>[2x]MFDNLTDRLSRTLRNISGRGRLTEDNVKDTLREVRMALLEADVALPVVREFINRVKEKAVGHEVNKSLTPGQEFVKIVRNELVAAMGEENQTLNLAAQPPAVVLMAGLQGAGKTTSVGKLGKFLREKHKKKVLVVSADVYRPAAIKQLETLAEQVGVDFFPSDVGQKPVDIVNAALKEAKLKFYDVLLVDTAGRLHVDEAMMDEIKQVHASINPVETLFVVDAMTGQDAANTAKAFNEALPLTGVVLTKVDGDARGGAALSIRHIT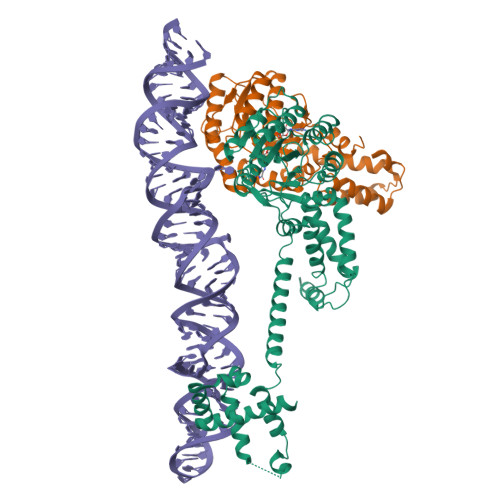GKPIKFLGVGEKTEALEPFHPDRIASRILGMGDVLSLIEDIESKVDRAQAEKLASKLKKGDGFDLNDFLEQLRQMKNMGGMASLMGKLPGMGQIPDNVKSQMDDKVLVRMEAIINSMTMKERAKPEIIKGSRKRRIAAGSGMQVQDVNRLLKQFDDMQRMMKKMKKG;>FARLKRSLLKTKENLGSGFISLFRGKKIDDDLFEELEEQLLIADVGVETTRKIITNLTEGASRKQLRDAEALYGLLKEEMGEILAKVDEPLNVEGKAPFVILMVGVNGVGKTTTIGKLARQFEQQGKSVMLAAGDTFRAAAVEQLQVWGQRNNIPVIAQHTGADSASVIFDAIQAAKARNIDVLIADTAGRLQNKSHLMEELKKIVRVMKKLDVEAPHEVMLTIDASTGQNAVSQAKLFHEAVGLTGITLTKLDGTAKGGVIFSVADQFGIPIRYIGVGERIEDLRPFKADDFIEALFARED[2x]> MIHELLLALSGYPGSIFTWNKRTGLQVSQDIPFLHPGETSVLNRLCKLGTDYIRFTEFIEQYTGHVQQQDHHPSQQGQVGLHGIYLRAFCRGLDSILQPYRQALLDLEQEFLADPHLSISHINYSLDQFHLLFPSIMVVVEQIKSQKIHGCQILETVYKHSCGGLPPVRSALEKTLAVCHGVMYKQLSAWMLHGLLLDQYEEFFVRQGSSSGNLAAAFEEEEDDLGIGGLTGKQLRELQDLRLIEEENMLAPSLKQFSLRAEMLPSYIPVRVAEKILFVGESVQMFENQNVNMSRTGSILKNQEDTFAAELHRLKQQPLFSLVDFESVLDRIRSTVAEHLWKLMVEESDLLGQLKIIKDFYLLGRGELFQAFIDVAQNMLKTPPTAVTEHDVNVAFQLSAHKVLLDDDNLLPLLNLTIDYHGKEHKDTSQPREGPFRDMSPREAPTSGWAALGLSYKVQWPLHILFTPAVLEKYNVVFKYLLSVRRVQSELQHCWALQMQRKHLESNKTDAIKWRLQNHMAFLVDNLQYYLQVDVLESQFSQLLQQINSTRDFESIRLAHDHFLSNLLAQSFILLKPVFHCLNEILELCHSFCSLVSQNLGPLDERGAGQLDILVKGFSCQSSLLFRILS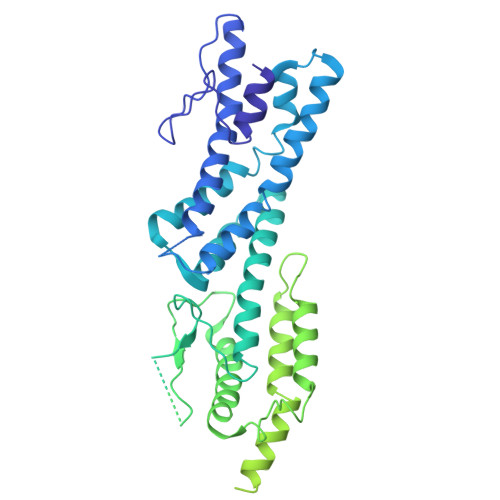SVRNHQINPDLAQLLLRLDYNKYYTQAGGTLGSFGL2-[(4-tert-butyl-3-nitrophenyl)carbonyl]-N-naphthalen-1-ylhydrazinecarboxamide 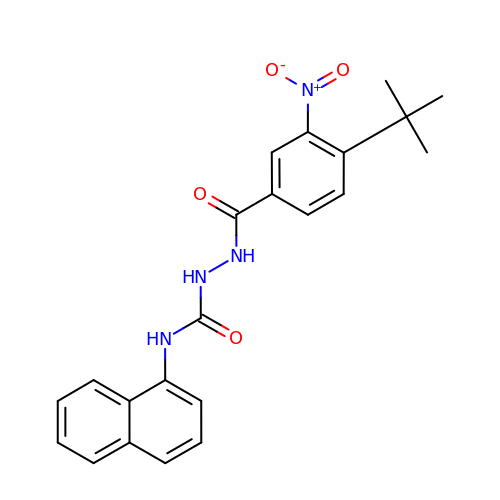| C22 H22 N4 O4 | YZMKNNITNHTADN-UHFFFAOYSA-N> MYK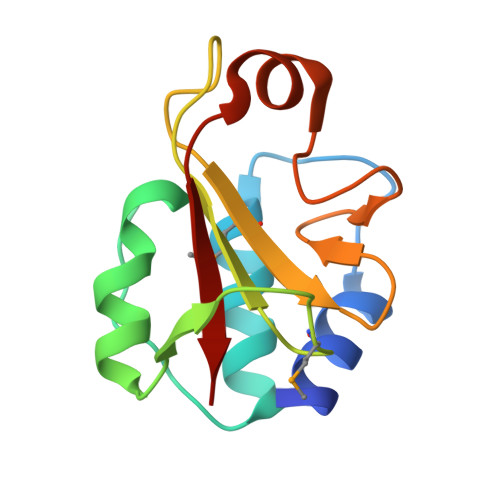GISAANYAASNIEPNSVGRCAEYVRKAIEWGGISLQRTRSAKDYGPSLLAAGFHEAIGSPMKGDVIVIQPAPGHPHGHMAIYDGSHWISDFKQLHGFYPGPAYRSAKPAYKTYRYH> MRVFIDEIARHVDQEVELRGWLYQRRSKGKIHFLILRDGTGFLQATVVQGEVPEAVFREADHLPQETALRVWGRVREDRRAPGGFELAVRDLQVVSRPQGEYPIGPKEHGID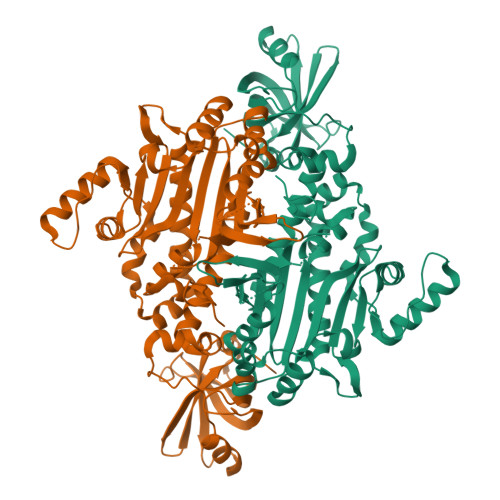FLMDHRHLWLRHRRPFAVMRIRDELERAIHEFFGERGFLRFDAPILTPSAVEGTTELFEVELFDGEKAYLSQSGQLYAEAGALAFAKVYTFGPTFRAERSKTRRHLLEFWMVEPEVAFMTHEENMALQEELVSFLVARVLERRSRELEMLGRDPKALEPAAEGHYPRLTYKEAVALVNRIAQEDPEVPPLPYGEDFGAPHEAALSRRFDRPVFVERYPARIKAFYMEPDPEDPELVLNDDLLAPEGYGEIIGGSQRIHDLELLRRKIQEFGLPEEVYDWYLDLRRFGSVPHSGFGLGLERTVAWICGLAHVREAIPFPRMYTRMRP>GGACUC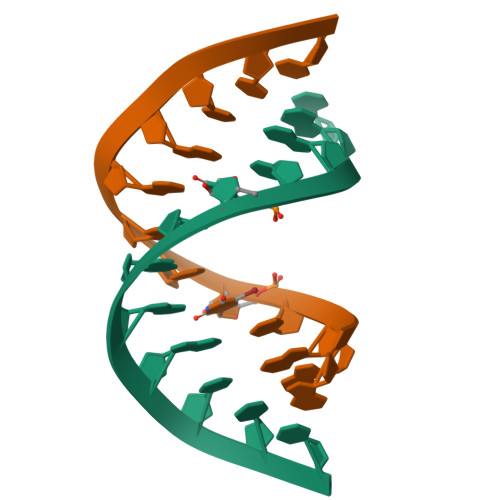GAGXCC[2x]>MVWLNGEPRPLEGKT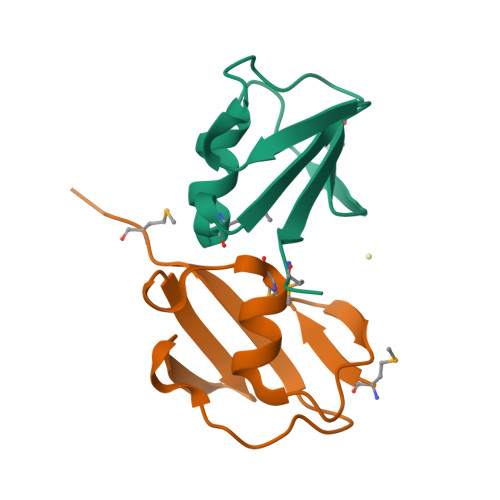LKEVLEEMGVELKGVAVLLNEEAFLGLEVPDRPLRDGDVVEVVALMQGG[2x]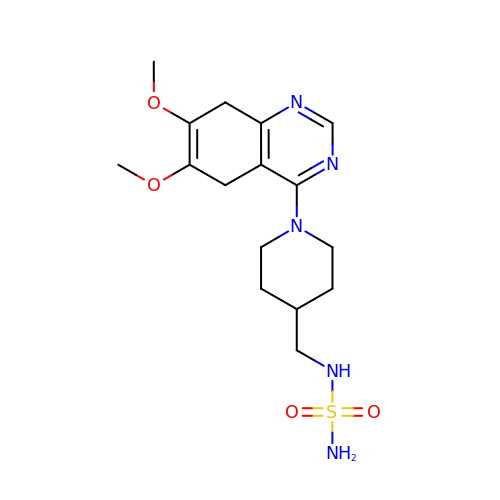N-{[1-(6,7-dimethoxy-5,8-dihydroquinazolin-4-yl)piperidin-4-yl]methyl}sulfuric diamide | C16 H25 N5 O4 S | FJBBCXRRTSLXGK-UHFFFAOYSA-N(4~{S})-4-[(1~{R})-1-[(1~{R},3~{a}~{S},4~{E},7~{a}~{R})-7~{a}-methyl-4-[2-[(3~{R},5~{R})-4-methylidene-3,5-bis(oxidanyl)cyclohexylidene]ethylidene]-2,3,3~{a},5,6,7-hexahydro-1~{H}-inden-1-yl]ethyl]-1-(4-hydroxyphenyl)octan-1-one | C35 H50 O4 | 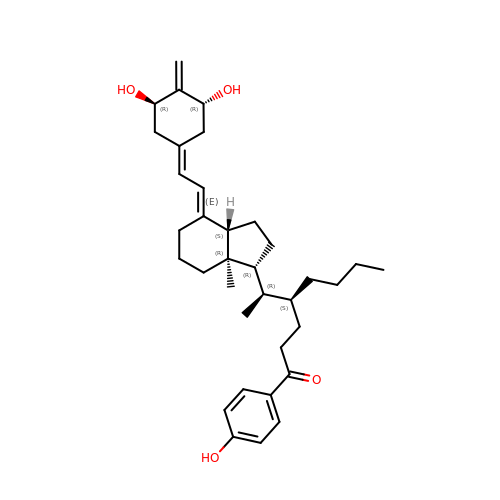IDKWEPILMVJEEL-HXCBKPQPSA-N>[2x]MAKLLIMSIVSFCFIFLLLLFFRYILKRYFNYMLNYKVWYLTLLAGLIPFIPIKFSLFKFNNVNNQAPTVESKSHDLNHNINTTKPIQEFATDIHKFNWDSIDNICTVIWIVLVIILSFKFLKALLYLKYLKKQSLYLNENEKNKIDTILFNHQYKKNIVIRKAETIQSPITFWYGKYIILIPSSYFKSVIDKRLKYIILHEYAHAKNRDTLHLIIFNIFSIIMSYNPLVHIVKRKIIHDNEVEADRFVLNNINKNEFKTYAESIMDSVLNVPFFNKNILSHSANGKKSLLKRRLINIKEANLKKQSKLILIFICIFTFLLMVIQSQFLMGQSITDYNYKKPLHNDYQILDKSKIFGSNSGSFVMYSMKKDKYYIYNEKESRKRYSPNSTYKIYLAMFGLDRHIINDENSRMSWNHKHYPFDAWNKEQDLNTAMQNSVNWYFERISDQIPKNYTATQLKQLNYGNKNLGSYKSYWMEDSLKISNLEQVIVFKNMMEQNNHFSKKAKNQLSSSLLIKKNEKYELYGKTGTGIVNGKYNNGWFVGYVITNHDKYYFATHLSDGKPSGKNAELISEKILKEMGVLNGQELALVPRGSSAHHHHHH

BlaR1 and MecR1 are membrane proteins with an N-terminal zinc metalloprotease domain and a C-terminal extracellular β-lactam-binding sensor domain. β-Lactam binding to the extracellular BlaR1 sensor domain regulates BlaI cleavage by the zinc metalloprotease domain in the cytoplasm. BlaR1 forms a domain-swapped dimer, with the zinc metalloprotease active site accessible from the cytoplasm. BlaR1 undergoes spontaneous autocleavage in cis between Ser283 and Phe284 and we describe the catalytic mechanism and specificity underlying the self and BlaI cleavage.

The structures of BlaR1(WT) and BlaR1(F284A) (the latter alone and in complex with ampicillin) were determined using cryo-electron microscopy (cryo-EM) to nominal resolutions of 3.8–4.6 Å. However, in the presence of ampicillin, we see a pronounced rigid body shift of about 6 Å to a position immediately abutting the membrane. The magnitude of this shift is consistent with the expected displacement of EL1 induced by the competitive binding of ampicillin. Thus, β-lactam binding and the consequent extrusion of EL1 from the active site appears to trigger movement of the sensor domain towards the outer leaflet of the membrane. Notably, a general compression parallel to the membrane normal was observed in the BlaR1(F284A)–ampicillin structure. Careful superposition of the reconstructions onto the re-entrant helices containing the catalytic HEXXH…E motif clearly demonstrates that structural elements on either side of the membrane are compressed towards each other in the presence of ampicillin. EL1 is situated immediately upstream of helix α3, which is observed kinked into the outer leaflet of the membrane as a result of the shift of EL1. Central to this is helix α3, which traverses the membrane directly linking EL1 and the metalloprotease domain. This helix is bent into the membrane at its N terminus in the BlaR1(F284A)–ampicillin structure, seemingly as a result of the force exerted on EL1 due to the acylation-induced sensor-domain movement. On the inner leaflet, concomitant motions are observed, with the metalloprotease domain drawn up to the membrane in the presence of ampicillin. Although a range of states exists in all of the samples, the equilibrium is shifted—BlaR1(WT) is dominated by a more extended conformation and the BlaR1(F284A)–ampicillin structure is more compact, with the sensor directly in contact with the outer leaflet of the membrane.N-[(1S)-1-[4-(2-fluorophenyl)-1H-imidazol-2-yl]-7,7-dihydroxy-7-(1,2-oxazol-3-yl)heptyl]-1-methylazetidine-3-carboxamide 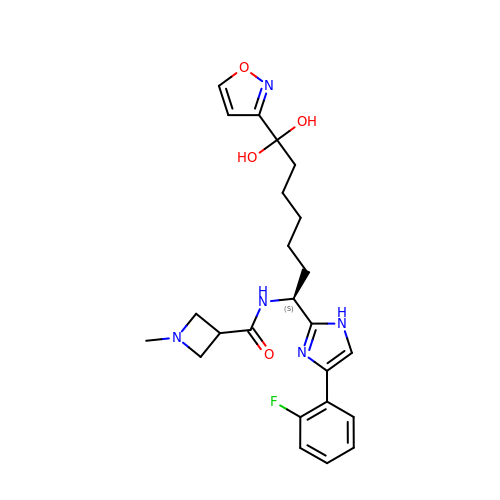| C24 H30 F N5 O4 | KTQGXHKWGKIKPU-IBGZPJMESA-N> GNPLRKFKLVFLGEQSVGKTSLITRFMYDSFDNTYQATIGIDFLSKTMYLEDRTVRLQLWDTAGLERFRSLIPSYIRDSTVAVVVYDITNVNSFQQTTKWIDDVRTERGSDVIIMLVGNKTDLADKRQVSIEEGERKAKELNVMFIETSAKAGYNVKQLFRRVAAALPGMESTQDRSREDMIDIKLEK;> EHLRLDNDQREKYIQEARNMGSTIRQPKLSNLSPSVIAQTNWKFVEGLLKECRNKTKRMLVEKMGREAVELGHGEVNITGVEENTLIASLCDLLERIWSHGLQVKQGKSALWSHLLHYQENRQRKLTSGSLSTSGILLDSERRKSDASAVMSPLRISLIQDMRHIQNIGEIKTDVGKARAWVRLSMEKKLLSRHLKQLLSDHELTKKLYKRYAFLRCDDEKEQFLYHLLSFNAVDYFCFTNVFTTILIPYHILIVPSKKLGGSMFTANPWICISGELGETQILQIPRNVLEMTFECQNLGKLTTVQIGHDNSGLYAKWLVECVMVRNEVTGHTYKFPCGRWLGKGMDDGSLERVLVGELLT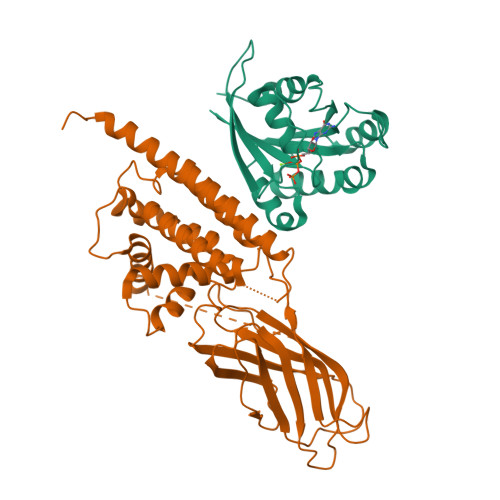SLPEVDERPCRTPPLQQSPSVIR> MAEHEQVNWPYVNTKLKRDPAVEAQIEKLLAKMTIEQKVAQMIQPEIGYLTVEQMRKYGFGSYLNGGNTAPYGNKRADQATWLKYADEMYLAAMDSTLDGIAIPTVWGTDAMHGH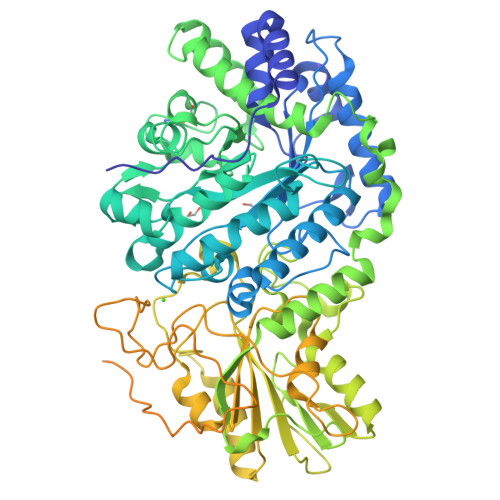SNVYGATLFPHNIGLGAARDTDLIKRIGQATAKEVAATGIEWSFAPTVAVVRDDRWGRTYESYSEDPDLVKRYAGEMVTGIQGDVGADFLKGSNRIATAKHFVGDGGTERGVDRGNTLIDEKGLRDIHSAGYFSAINQGVQSVMASFNSWNGKRVHGDKHLLTDVLKNQLGFDGFVVSDWNAHKFVEGCDLEQCAQAINAGVDVIMVPEHFEAFYHNTVKQVKAGVIAESRINDAVRRFLRAKIRWGVFTKSKPSARPESQHPQWLGAAEHRTLAREAVRKSLVLLKNNESILPIKASSRILVAGKGANAINMQAGGWSVSWQGTDNTNSDFPNATSIFSGLQSQVTKAGGKITLSESGEYTSKPDVAIVVIGEEPYAEWFGDIELLEFQHETKHALALLKQLKADNIPVVTVFLSGRPLWVNKELNASDAFVAAWLPGSEGEGVADVLLTNKQGKTQFDFTGKLSFSWPKYDDQFTLNLNDADYDPLFAYGYGLTYQDNINVPVLSEKTSPKKTVNSDSHPLFVRSLAKNMTWQLADTSTQKVLASGASATSGDKQSLLMQSVNLSYAEDGRGFNWRAQAALSLSYLEPTPLDSKFSTGYLELKMRIDKAPEQGANLQVMCSESNCLRDIDFSSFSQLMADKSWHTLAIPLHCDDSDQAEQPITDALRITSQNLSLAIADVALTIKPSDDSISLTCAKLEHHHHHH1-(5-BROMO-1-BENZOTHIOPHEN-3-YL)METHANAMINE 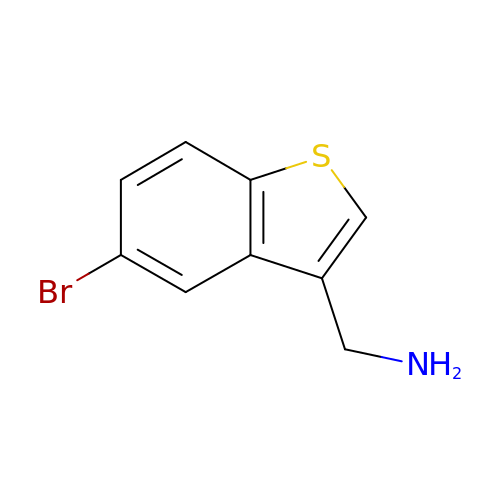| C9 H8 Br N S | DVYWOASQESEKEC-UHFFFAOYSA-N> MTEQRPLTIALVAGETSGDI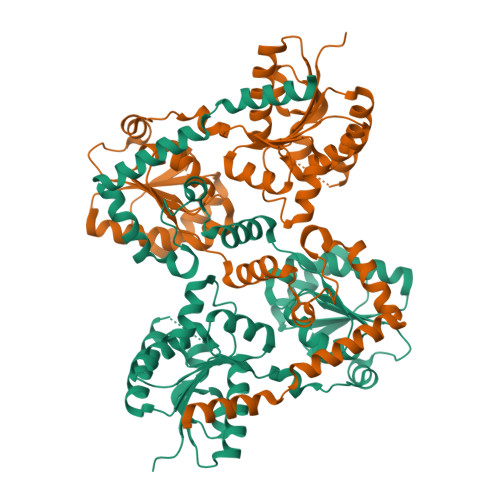LGAGLIRALKEHVPNARFVGVAGPRMQAEGCEAWYEMEELAVMGISESSGRSRRSSHIRADLTKRFGELKPDVFVGIDAPDFNITLEGNLKKQGIKTIHYVSPSVWAWRQKRVFKIGRATDLVLAFLPFEKAFYDKYNVPCRFIGHTMADAMPLDPDKNAARDVLGIPHDAHCLALLPGSRGAEVEMLSADFLKTAQLLRQTYPDLEIVVPLVNAKRREQFERIKAEVAPDLSVHLLDGMGREAMVASDAALLASGTAALECMLSKCPMVVGYRMKPFTFWLAKRLVKTDYVSLPNLLAGRELVKELLQEECEPQKLAAALLPLLANGKTSHAMHDTFRELHQQIRCNADEQAAQAVLELAQ> MLGITSALLCVTAGRAALVASELQKLVPVLLPLLDPPIAKGVNVSAAQLIVASGHTSRRNDVHLPDCPVMAHALPLTALAEHSAFLRHPCRACLKRRVHFLSSEHFCMHLEEKCSQGGGGMPAEWESIAAGQFGLFTHFTDEFVMYATSRREPGWTWLVYDKERPEGHRLVVVNFPANRVPLVLGLWPLAVINMTESRLLSAIGARTKTSAAESSPAPWSRAARNPLVAEASTATVAAMAAAVTDTVDGLDGSLSS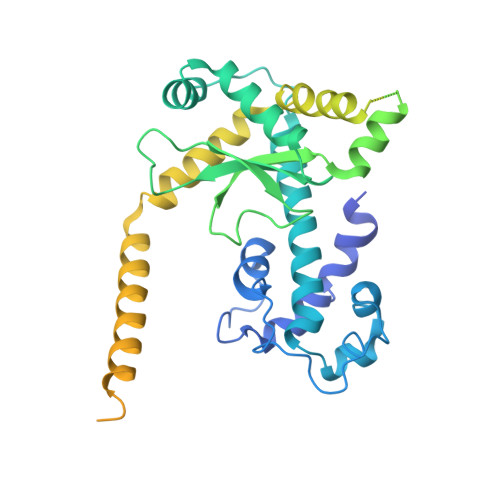IRAQVAQEAVLKMNWGFVLQQWKQAESYYESAERERKVQAQRTKMEREAALAEMSKLRDSGATILTSDTVEITVAGSDAVPEKASRDLKASTQTTKEPRKEEEETAGVGTANQDPHCTQLEDGTWQYAYKNGDLTLLRPDGTRVFKKSDLTTTVFADGSTLYEYPNKTSILDRVDGVRVTTFADGTTKEGRYK>[18x]MPQEARTPQQQVTADEVGDWYDKFGEVYHLTLGESVHCGLWFPPDAPVPQDMELVTMSSQAQDRYTDYLIETLDPKAGQHLLDIGCGTGRTALKAARQRGIAVTGVAVSKEQIAAANRLAAGHGLTERLTFEVAD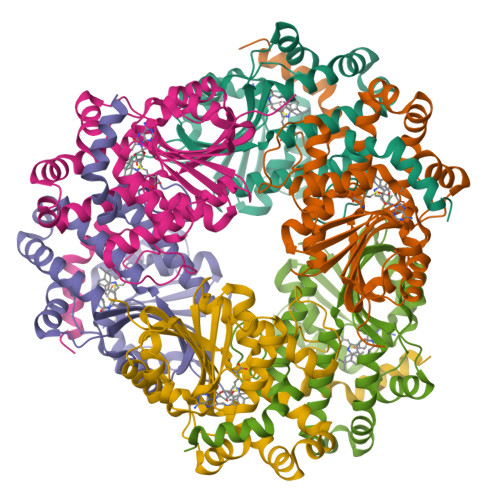AMRLPYEDESFDCAWAIESLCHMDRAKALGEAWRVLKPGGDLLVLESVVTEELTEPETALFETLYAANVPPRLGEFFDIVSGAGFHTLSLKDLSANLAMTMNVFALGVYSRRAEFTERFGAEFVDGLLAGLGSAQETLIRKTRFFMATLRKPAVLEHHHHHH>GGSGGSYRVVAYYISWGAYGRSYFPSDIDYSKVTHINYAFANIKDGEVVVGDPGVDDGGKNNFTALRKAKKAHPHLRNLISVGGWSWSSGFSDAAATPEARKRFADSAVAFIRKYGFDGVDIDWEYPVEGGAENMKHRPEDKQNYTLLTRSLREALDTAGKADGKYYELTTAVWGNDKFIANTEMDKVSRDFDFINVMSYDFNGTWNKFSGHNAPFVNDPAYDKPGIGKTFNVVSAVEAYLKAGVPADKLVVGVPLYGYSWKGCAAGERNGEYQDCNGKGRGTWEDGNLDFTDIEKNLLNKKGFKRYWNDTAKAAYLYNAETGEFVTYEDPQALKIKLDYIKSKGLGGAMYWEITADRKQ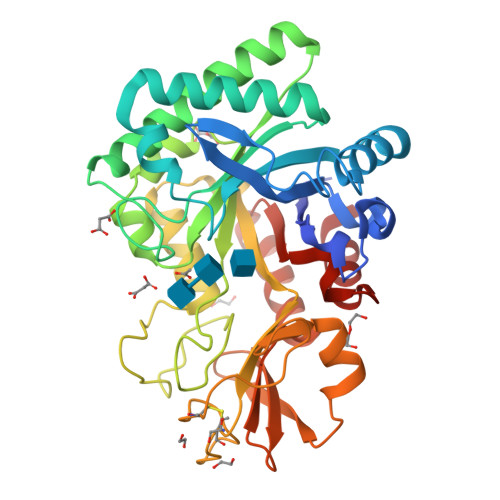TLVNLIADELLT[2x]Transition metal transporting P-type (PIB) ATPase proteins are critical for cellular heavy-metal homeostasis, providing efflux of for example copper, zinc, and cobalt from the intracellular milieu. The PIB-ATPases belong to the P-type ATPase superfamily of integral membrane proteins, which exploit energy from ATP hydrolysis for transport of cargo across cellular membranes. Here, we present structures and complementary functional analyses of an archetypal PIB-4-ATPase, sCoaT from Sulfitobacter sp. NAS14-1. The sCoaT structures reveal that PIB-4-ATPases comprise soluble A-, P-, and N-domains, shown in yellow, blue, and red, respectively, as well as a transmembrane domain with eight helices: MA and MB, in cyan, and M1–M6, in grey, and that the PIB-4-topology lacks classical so-called heavy-metal-binding domain.

We determined structures of sCoaT in metal-free conditions supplemented with two different phosphate analogues, BeF3− and AlF4−, respectively, which previously have been exploited to stabilize E2 reaction intermediates of the transport cycle of PIB-ATPases. The structures were determined at 3.1 and 3.2 Å resolution, using molecular replacement (MR) as phasing method and SsZntA as search model, and the final models yielded R/Rfree of 24.4/26.8 and 21.8/25.5. (a) sCoaT E2-AlF4− (P21212, with one molecule per asymmetric unit). The classical view of P-type ATPases is that the E2P state is outward open and that the following transition state of dephosphorylation, E2.Pi, is occluded, and that these conformations can be stabilized using the phosphate analogues employed here for structure determination, BeF3− and AlF4−, respectively. Surprisingly however, analysis of the two obtained structures suggests that the anticipated significant domain reorientations are absent in sCoaT, and the models are in contrast rather similar. The compact assembly of the soluble domains and the position of the A-domain near the P-domain, placing the conserved TGE motif responsible for dephosphorylation towards the phosphorylation site, are typically associated with commencement of dephosphorylation, indicating that the two structures are trapped in an E2.Pi like transition state. Alignment of the E2-BeF3− and E2-AlF4− structures of sCoaT demonstrates that they are very similar (RMSD = 1.1), and comparison to the equivalent structures of SsZntA support the conclusion from (a–d) that both structures have been captured in occluded E2.Pi transition states. The E2-BeF3− and the E2-AlF4− (not shown) structures are occluded, lacking continuous connection between the ion-binding site to the outward environment. The rigid conformation observed for H657 in the E2-BeF3− structure is also observed in the E2-AlF4− structure. The M-domain is in general less well resolved than the soluble domains, and the domain is somewhat more well resolved in the E2-BeF3− structure than in E2-AlF4− structure.

> MRKVVADLNAVEEENMPENHTPDDGHNHAHGGFLNRILGGRAEVIFAVLCGICLLLGWLGPKYGIMSEQFGFGLLLAAYFFGGYFTLREAVEKISKGQFQIDFLMLVAASGAAILGEWAEGAFLLFLFSVGHALENYAMGRARNAVAALAGLTPDEALVRRGDKTETVLIENLLVGDIVVVRSNERLPADGFVVKGSSAVNQAPITGESAPVDKLPVDDPEFAAANLDKLTPQTRVFAGSINGSGSLDVQVTKLSGESTLARVVTLVAEAQTRQSPTQNFTKKFEKIFVPCVIALAFVTSFSFLILDETAAQSFYRAMAVLVAASPCALAIATPSAVLSGVARAARGGVLIKGGAPLEAMGHLDAIAFDKTGTLTIGEPHLVEITPYGDATETELLQVSAAVEMLSDHPLAQAVVRDVKDRLGDLPSEASDFANIIGQGVSAKVDSKVVHIGKTALFESVAGLPLPDDLRGTVEAMSQNGRTTMIVRSGDRYLGAIGLMDTPREDARSVIAALRDLGLKRMMMISGDNQNVANAVAKEVGLDTAFGDLMPEDKVTKIAALKADGGVAMVGDGVNDAPAMANATVGIAMGAAGSDVALETADIALMADDLQTLPFAVGLSRKTSRIIRLNLWFSLGVVALLIPATLFGLGIGPAVLVHEGSTLVVVANALRLLAFKDNRVKSA>GSDEDTYYLQVRGRRNFEILMELKRSLELMELVPQPL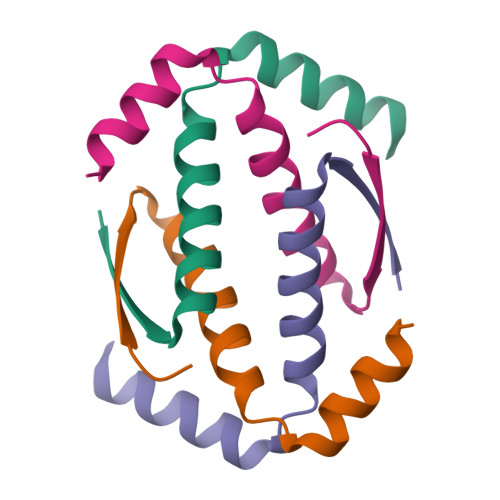VDSYDQQQQLLQR[2x]> MGGSVAAQDEFYRSGWALNMKELKLLQTIGKGEFGDVMLGDYRGNKVAVKCIKNDATAQAFLAEASVMTQLRHSNLVQLLGVIVEEKGGLYIVTEYMAKGSLVDYLRSRGRSVLGGDCLLKFSLDVCEAMEYLEGNNFVHRDLAARNVLVSEDNVAKVSDFGLTKEASSTQDTGKLPVKWTAPEALREKKFSTKSDVWSFGILLWEIYSFGRVPYPRIPLKDVVPRVEKGYKMD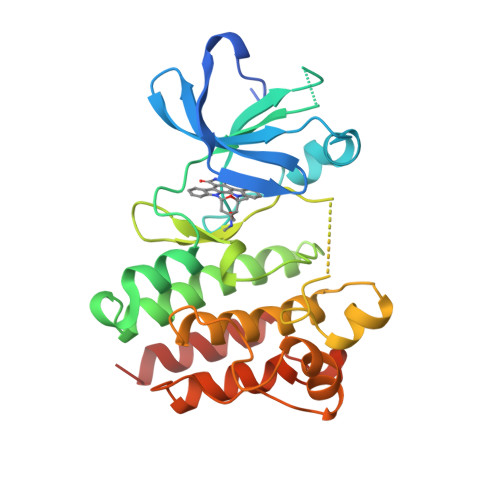APDGCPPAVYEVMKNCWHLDAAMRPSFLQLREQLEHIKTHELHL>SQYALARTFATQKVSLEESVLSQVTTAIQTAQEKIVYAGNGTLSDDDRASLATDLQGIRDQLMNLANSTDGNGRYIFAGYKTEAAPFDQATGGYHGGEKSVTQQVDSAITLEIGHTGAQIFNSICECAVPEPDGSDSEKNLFVMLDTAIAALKTP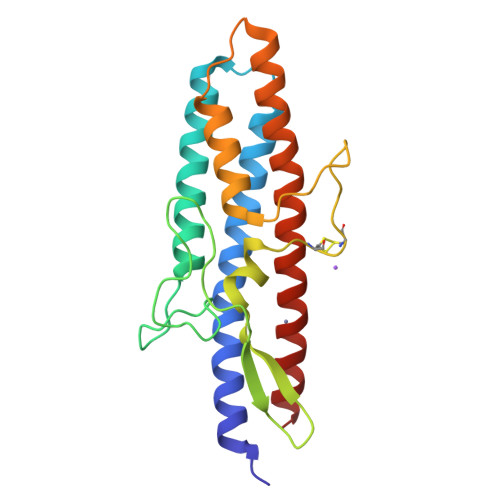VEGNNVEKEKAAAAIDKTNRGLKNSLHNVLEVRWELEWFLELLSAK[2x]> MDLTVEPNLHSLITSTTHKWIFVGGKGGVGKTTSSCSIAIQMALSQPNKQFLLISTDPAHNLSDAFGEKFGKDARKVTGMNNLSCMEIDPSAALKDMNDMAVSRANNNGSDGQGDDLGSLLQGGALADLTGSIPGIDEALSFMEVMKHIKRQEQGEGETFDTVIFDTAPTGHTLRFLQLPNTLSKLLEKFGEITNKLGPMLNSFMGAGNVDISGKLNELKANVETIRQQFTDPDLTTFVCVCISEFLSL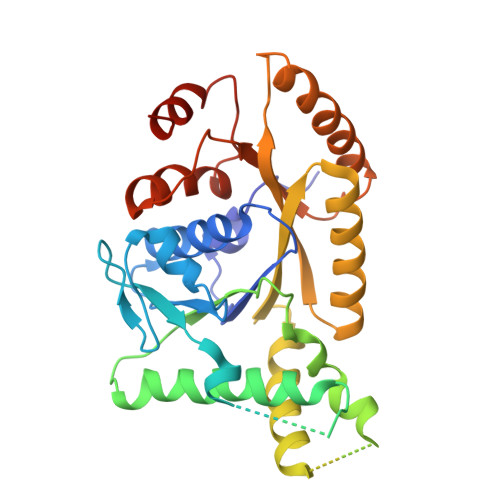YETERLIQELISYDMDVNSIIVNQLLFAENDQEHNCKRCQARWKMQKKYLDQIDELYEDFHVVKMPLCAGEIRGLNNLTKFSQFLNKEYNPITDGKVIYELEDKELEHHHHHH>SNAQITDGKQYITLDKPIAGEPQVLEFFSFYCPHCYQFEEVLHVSDNVRQKLPEGTKMTKYHVEFLGPLGKDLTQAWAVAIALGVEDKITAPMFEAVQKTQTVQSVADIRKVFVDAGVKGEDYDAAWNSFVVKSLVAQQEKAAADLQLQGVPAMYVNGKYQLNPQGMDTSNMDVFVAQYADTVKQLVEKK[6x]

Typically, the oxidative folding machinery includes a soluble thioredoxin-fold protein, DsbA, and an integral membrane protein partner, DsbB. The disulfide form of DsbA is highly oxidizing and donates its disulfide bond to unfolded substrate proteins, leaving DsbA in the inactive reduced form. The inner membrane protein DsbB, in concert with its cofactor ubiquinone, interacts with reduced DsbA to oxidize the active site cysteines and convert DsbA to its functionally competent disulfide form. We determined the high resolution crystal structure of reduced KpDsbA and the NMR solution structure of oxidized KpDsbA, and we measured the redox properties of this enzyme.

The asymmetric unit contains six KpDsbA molecules each adopting the typical DsbA fold. Structural superposition of these six independent copies yielded a root mean square deviation (RMSD) < 0.45 Å for 176 Cα atoms between residues Gly6 - Val181. The cysteine residues (Cys30 and Cys33) are present in the reduced state in the crystal structure. The six independent copies of KpDsbA in the crystal structure allow an analysis of conformational variability of the loop residues forming the binding surface. The side chain variations do not influence the surface accessibility of the hydrophobic groove, which was calculated to be 371 ± 32 Å2 by CastP across the 6 molecules. Moreover, the hydrophobic nature of the groove is unaffected by the side chain conformational variability as indicated by the proportion of carbon atoms lining this groove (69 ± 3 %). The overall conformation of the NMR structure of oxidized KpDsbA is similar to that of the crystal structure of reduced KpDsbA. For example, superposition of molecule A in the crystal structure of reduced KpDsbA with the first structure in the NMR ensemble of oxidized KpDsbA, yields an RMSD of 1.09 Å over 169 Cα atoms. As expected, the redox properties, surface characteristics and binding properties of KpDsbA are similar to those of EcDsbA suggesting that inhibitors developed against EcDsbA are likely to also be effective against other members of this DsbA subclass. By contrast, the six molecules in the asymmetric unit of KpDsbA crystal structure is far from ideal for rapid fragment-screening, but is nevertheless advantageous for follow up analysis.> MTLAILAVFSVALTLLGFVLPPQGVKRATLLGLALALASLLLTWGKPFAFGPYAVDGVSQVFTLLALLGALWTVGLVRSGRFEFYLLVLYAALGMHLLASTRHLLLMLVALEALSLPLYALATWRRGQGLEAALKYFLLGALAAAFFLYGAALFYGATGSLVL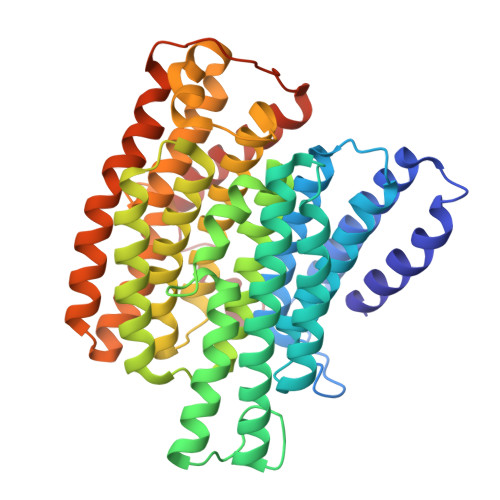GAPGEGPLYALALGLLLVGLGFKAALAPFHFWTPDVYQGSPTPVVLFMATSVKAAAFAALLRVAAPPEALALLVALSVVVGNLAALAQKEAKRLLAYSSIAHAGYMALALYTGNAQALGFYLLTYVLATGLAFAVLSQISPDRVPLEALRGLYRKDPLLGLAFLVAMLSLLGLPPLAGFWGKYLAFAEAARAGAWGVLVLALVTSAVSAYYYLGLGLAVFARPEETPFRPGPPWARAAVVAAGVLLLALGLLPGLVLPALAAGG> ARSTNTFNYATYHTLDEIYDFMDLLVAEHPQLVSKLQIGRSYEGRPIYVLKFSTGGSNRPAIWIDLGIHSREWITQATGVWFAKKFTEDYGQDPSFTAILDSMDIFLEIVTNPDGFAFTHSQNRLWRKTRSVTSSSLCVG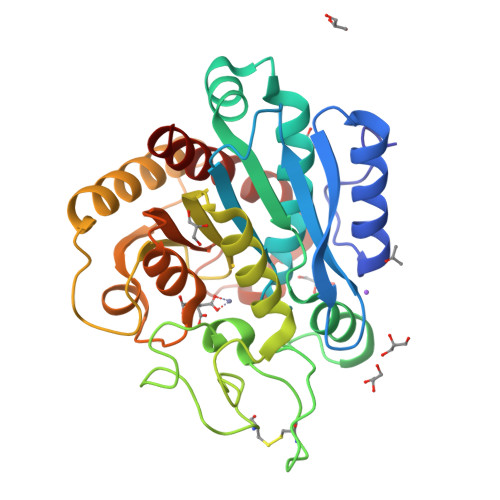VDANRNWDAGFGKAGASSSPCSETYHGKYANSEVEVKSIVDFVKDHGNFKAFLSIHSYSQLLLYPYGYTTQSIPDKTELNQVAKSAVEALKSLYGTSYKYGSIITTIYQASGGSIDWSYNQGIKYSFTFELRDTGRYGFLLPASQIIPTAQETWLGVLTIMEHTLNNLY>[4x]GHMTKTKFEKVLLIVNPKAGQGDLHTNLTKIVPPLAAAFPD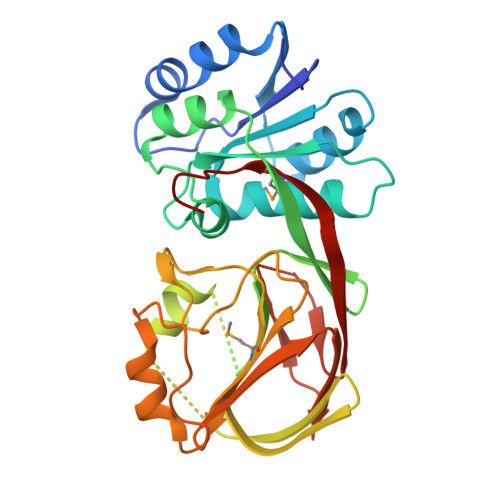LHILHTKEQGDATKYCQEFASKVDLIIVFGGDGTVFECTNGLAPLEIRPTLAIIPGGTCNDFSRTLGVPQNIAEAAKLITKEHVKPVDVAKANGQHFLNFWGIGLVSEVSNNIDAEEKAKLGKIGYYLSTIRTVKNAETFPVKITYDGQVYEDEAVLVMVGNGEYLGGIPSFIPNVKCDDGTLDIFVVKSTGIQAFKDYIGKKLFEDSNENDIFHVKAKSIHIETEEEKEVDTDGESSLHTPCQIELLQGHFTMIYNPAVVGS>MAPSRLCVYCADVCPDRLRCAAWLLATGIFLLLAGCSEAKAPTALERVQKEGVLRVITRNSPATYFQDRNGETGFEYELAKRFAERLGVELKIETADNLDDLYAQLSREGGPALAAAGLTPGREDDASVRYSHTYLDVTPQIIYRNGQQRPTRPEDLVGKRIMVLKGSSHAEQLAELKKQYPELKYEESDAVEVVDLLRMVDVGDIDLTLVDSNELAMNQVYFPNVRVAFDFGEARGLAWALPGGDDDSLMNEVNAFLDQAKKEGLLQRLKDRYYGHVDVLGYVGAYTFTQHLQQRLPRYESHFKQSGKQKDTDWRLLAAIGYQESLWQPGATSKTGVRGLMMLTNRTAQAMGVSNRLDPKQSIQGGSKYFVQIRSELPESIKEPDRSWFALAAYNIGGAHLEDARKMAEKEGLNPNKWLDVKKMLPRLAQKQWYAKTRYGYARGGET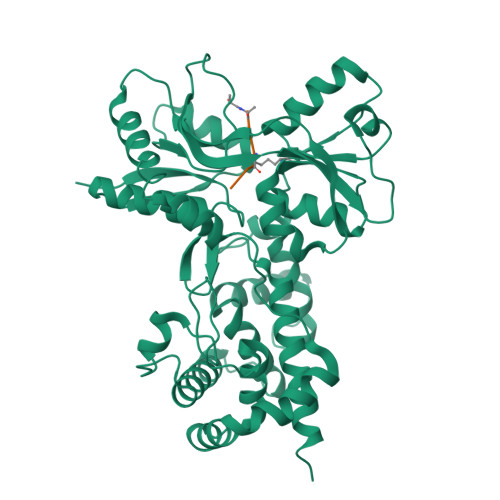VHFVQNVRRYYDILTWVTQPQMEGSQIAESGLHLPGVNKTRPEEDSGDEKL[4x];> XAEKAA> MVSKGEEDNMASLPATHELHIFGSINGVDFDMVGQGTGNPNDGYEELNLKSTKGDLQFS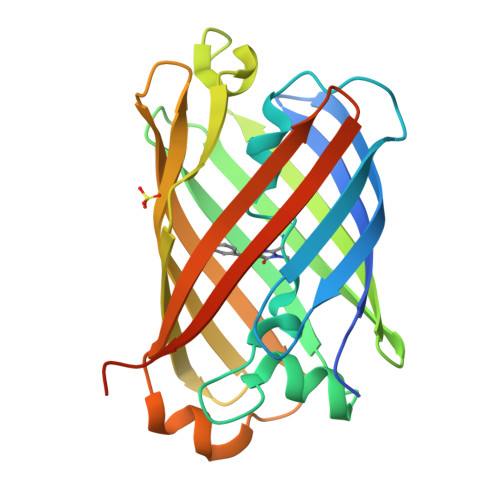PWILVPHIGYGFHQYLPYPDGMSPFQAAMVDGSGYQVHRTMQFEDGASLTVNYRYTYEGSHIKGEAQVKGTGFPADGPVMTNSLTAADWCRSKKTYPNDKTIISTFKWSYTTGNGKRYRSTARTTYTFAKPMAANYLKNQPMYVFRKTELKHSKTELNFKEWQKAFTDVMGMDELYKHHHHHH> MDLVLLEKALLGLFAAAVLAVAVAKLTGKRYRLPPGPAGAPVVGNWLQVGDDLNHRNLMSLAKRFGDIFLLRMGVRNLVVVSTPELAKEVLHTQGVEFGSRTRNVVFDIFTGKGQDMVFTVYGDHWRKMRRIMTVPFFTNKVVAQNRVGWEEEARLVVEDVRKDPRAAAEGVVIRRRLQLMMYNDMFRIMFDTRFESEQDPLFNKLKALNAERSRLSQSFEYNYGDFIPVLRPFLRGYLNRCHDLKTRRMKVFEDNFVQERKKVMAQTGEIRCAMD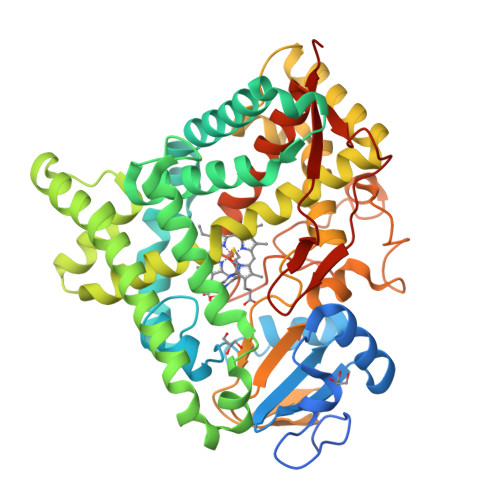HILEAERKGEINHDNVLYIVENINVAAIETTLWSIEWGIAELVNHPAIQSKLREEMDSVLGAGVPVTEPDLERLPYLQAIVKETLRLRMAIPLLVPHMNLNDGKLAGYDIPAESKILVNAWFLANDPKRWVRPDEFRPERFLEEEKTVEAHGNDFRFVPFGVGRRSCPGIILALPIIGITLGRLVQNFQLLPPPGQDKIDTTEKPGQFSNQIAKHATIVCKPLEAHHHHHH> QVTPRPEAAPGARPGFRAPARIISPEIMPDNKVTFRVYSKDASKVTITGEWQTGPGGVEELVKNDTGMFSITVGPLKPELYAYNFTVDGVKALDANNV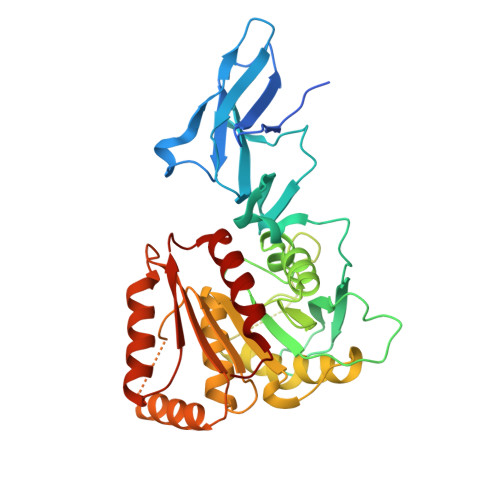QVRRDGTNYQNFFIIPGPESDLYFHKNNVPHGTVTKVWYKSSVIGFDRRMYVYTPAGYEGDTQRYPVFYLLHGAGGDEDAWTNMGRTAQIMDNLIAQGKAKPMIVVMTNGNANQAGAQNEVPPVPVTQGQQGIPSGSGMTGKFEEHLVKDVVPFIEKNFRALTGKDNRAIAGLSMGGGHTQTITNDNPGMFSYIGVFSMGIMAGRQQGADAEKIEKERDAKIEALKKSGYKLYWIACGKDDFVYQSALTLRNTLDKHNFKYVYRESTGGHTWANWRIYLSEFAPMLFKLL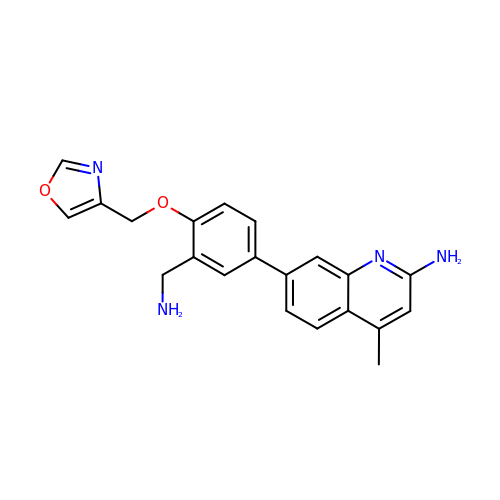7-{3-(aminomethyl)-4-[(1,3-oxazol-4-yl)methoxy]phenyl}-4-methylquinolin-2-amine | C21 H20 N4 O2 | JUUSNAFIFJKARW-UHFFFAOYSA-N> MEGAKPTLQLVYQAVQALYHDPDPSGKERASFWLGELQRSVHAWEISDQLLQIRQDVESCYFAAQTMKMKIQTSFYELPTD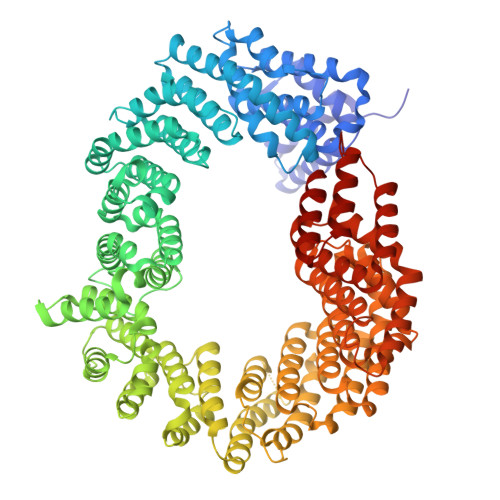SHASLRDSLLTHIQNLKDLSPVIVTQLALAIADLALQMPSWKGCVQTLVEKYSNDVTSLPFLLEILTVLPEEVHSRSLRIGANRRTEIIEDLAFYSSTVVSLLMTCVEKAGTDEKMLMKVFRCLGSWFNLGVLDSNFMANNKLLALLFEVLQQDKTSSNLHEAASDCVCSALYAIENVETNLPLAMQLFQGVLTLETAYHMAVAREDLDKVLNYCRIFTELCETFLEKIVCTPGQGLGDLRTLELLLICAGHPQYEVVEISFNFWYRLGEHLYKTNDEVIHGIFKAYIQRLLHALARHCQLEPDHEGVPEETDDFGEFRMRVSDLVKDLIFLIGSMECFAQLYSTLKEGNPPWEVTEAVLFIMAAIAKSVDPENNPTLVEVLEGVVRLPETVHTAVRYTSIELVGEMSEVVDRNPQFLDPVLGYLMKGLCEKPLASAAAKAIHNICSVCRDHMAQHFNGLLEIARSLDSFLLSPEAAVGLLKGTALVLARLPLDKITECLSELCSVQVMALKKLLSQEPSNGISSDPTVFLDRLAVIFRHTNPIVENGQTHPCQKVIQEIWPVLSETLNKHRADNRIVERCCRCLRFAVRCVGKGSAALLQPLVTQMVNVYHVHQHSCFLYLGSILVDEYGMEEGCRQGLLDMLQALCIPTFQLLEQQNGLQNHPDTVDDLFRLATRFIQRSPVTLLRSQVVIPILQWAIASTTLDHRDANCSVMRFLRDLIHTGVANDHEEDFELRKELIGQVMNQLGQQLVSQLLHTCCFCLPPYTLPDVAEVLWEIMQVDRPTFCRWLENSLKGLPKETTVGAVTVTHKQLTDFHKQVTSAEECKQVCWALRDFTRLFR>[4x]MSEQNNTEMTFQIQRIYTKDISFEAPNAPHVFQKDWQPEVKLDLDTASSQLADDVYEVVLRVTVTASLGEETAFLCEVQQGGIFSIAGI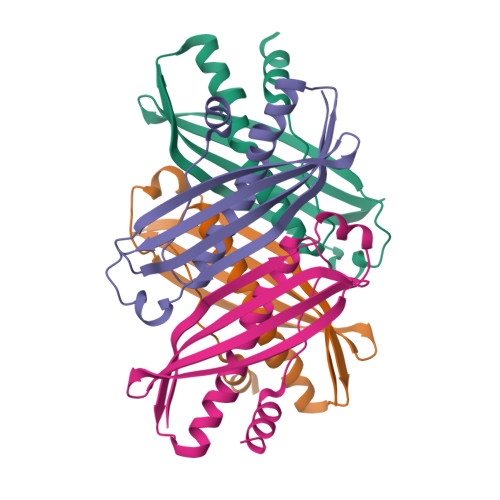EGTQMAHCLGAYCPNILFPYARECITSMVSRGTFPQLNLAPVNFDALFMNYLQQQAGEGTEEHQ> MGYQPPSDYKQCKHLKSFPVSELKGDNKELWLMKVPANIDISQLKSLPLDTDATVSTVELGSKNFNVLQNTSTQEGSDNTNLSL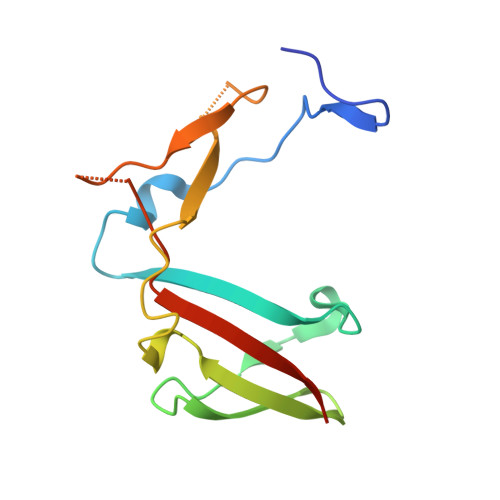LIPSEKKKETLKVATSKDNKSVYFDRVFTISETARIP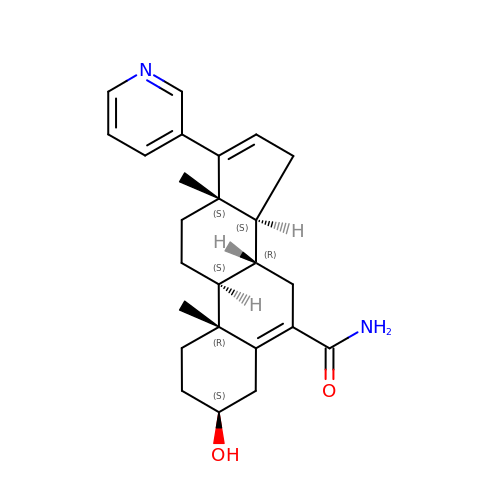3-hydroxy-17-(3-pyridyl)-androst-5,16-dien-6-amide | C25 H32 N2 O2 | CPGOQTKJUPLDPD-ACAUBTHISA-N> MVSAIVLYVLLAAAAHSAFAAMVHHHHHHSAEETLMDSTTATAELGWMVHPPSGWEEVSGYDENMNTIRTYQVCNVFES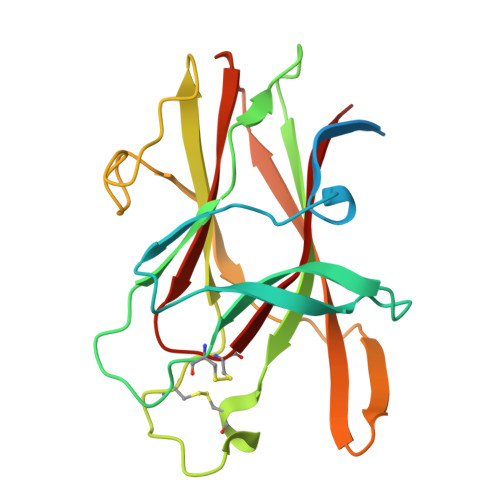SQNNWLRTKFIRRRGAHRIHVEMKFSVRDCSSIPSVPGSCKETFNLYYYEADFDSATKTFPNWMENPWVKVDTIAADESFSQVDLGGRVMKINTEVRSFGPVSRSGFYLAFQDYGGCMSLIAVRVFYRK The tRNAHis guanylyltransferase (Thg1) family comprises enzymes from all three domains of life, all of which catalyze reverse addition (3′–5′) of nucleotides to polynucleotide substrates. Here we report the first crystal structure of any TLP, that of the gram-positive soil bacterium Bacillus thuringiensis (BtTLP). Similar to yeast and human Thg1, BtTLP is a tetramer consisting of a dimer of dimers. In contrast to eukaryotic Thg1 enzymes, TLP enzymes prefer to catalyze repair of tRNAs with damaged 5′-ends, making them well-suited to participating in tRNA quality control pathways in vivo.

In the BtTLP/GTP complex a GTP molecule is observed in the activation site for all four monomers, bound in a similar orientation to the dGTP nucleotide in the hTHG1/dGTP complex. A second complete GTP is seen in two of the four subunits of the BtTLP tetramer (monomers A and B), with a second partial GTP observed for monomers C and D.. The amide of D46 participates in a hydrogen bond with O6 of guanine, and the carbonyl moiety of A42 interacts with N1, identical contacts to those observed in the hTHG1/GTP structure. In the BtTLP/GTP structure, however, there are additional contacts between T38 and the bound GTP, with main chain carbonyl-N2 and OG1-N3 interactions provided by this residue. Interestingly, K43 does not interact with the guanine base in the BtTLP GTP-bound structure, as there would likely be a steric clash between the lysine side chain and the exocyclic amine of the base. In contrast to the hTHG1/dGTP structure where the second bound dGTP nucleotide was highly disordered so that only the 5′-triphosphate moiety was visible in the electron density map, the GTP-bound BtTLP structure reveals complete density for the second nucleotide. The α-phosphate forms a salt bridge with R28 and K99′ (of the adjacent monomer in the dimer). The γ-phosphate participates in salt bridges with three residues: R131, R16′, and K99′. In the BtTLP structure, however, the carboxylate group of E12 participates in salt bridge interactions with two arginines, R28 and R131, both of which contact the triphosphate tail of the GTP in the nucleotide transfer site. In the BtTLP structure, however, the side chain of the third carboxylate, E76, is located roughly 4 Å away from the aliphatic chain of R28, a residue shown to be important in binding the incoming GTP molecule.

>[4x]MDSIGDRMKRYENAYRIKLPERMPVIVRIDGAHFHTYTKGCAKPFDQDLAEAFWETCKYLAQNIMGAKLVYHQSDEISILITNYDKLTTQSWFENNLQKIASVSASMATAKFNEVMREKYPDKPLATFDGRAQVLPQDEVANYFIWRQQDASKNSISMVAQANFPHKQLQGLNGKDMQDKLMTEKNINWNDLPVWQKRGICIIKEFYEKNGALRSRWSVDHETPIISKDREYVEQFVYLNRGAAA> MKKQYLKSGSGTRKEKDKAKRWFLDNGSIFLREL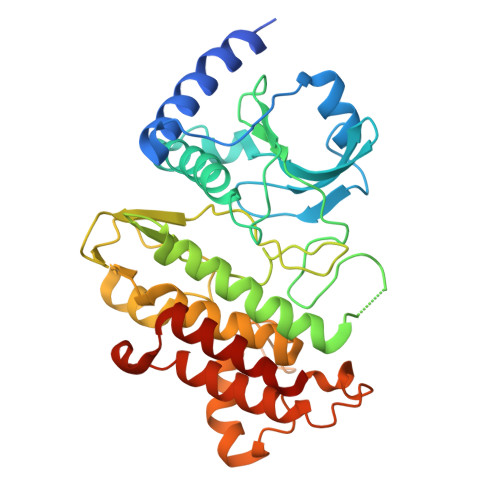VADCNGKSIPIRSFSPEQILKATNNFDSSCFVSQDVYYKWYRGEIEDRSYMIKRFSEDEITGKRHRVKEVYNDIVLSARMSNHSNFLQLLGCCLEFPFPVLVFEFAEHGAMNQRGGVIVNGEESLLPWSVRLKIGKEIANAVTYLHTAFPKIIIHRDVKPMHVFLDKNWTAKLSDLSFSISLPEGKSRIEAEWVLGTFGYIDPLYHKTCFVTEYTDVYSFGICLLVIITGKPAIMTISDGDLQGILSLVRELCENGKLDEVIDPRLMKDITSGQRLQVEACVVLALRCCKERDEDRPKMIQVAKELKQIEASLKNSS> MQNNNEFKIGNRSVGYNHEPLIICEIGINHEGSLKTAFEMVDAAYNAGAEVVKHQTHIVEDEMSDEAKQVIPGNADVSIYEIMERCALNEEDEIKLKEYVESKGMIFISTPFSRAAALRLQRMDIPAYKIGSGECNNYPLIKLVASFGKPIILSTGMNSIESIKKSVEIIREAGVPYALLHCTNIYPTPYEDVRLGGMNDLSEAFPDAIIGLSDHTLDNYACLGAVALGGSILERHFTDRMDRPGPDIVCSMNPDTFKELKQGAHALKLARGGKKDTIIAGEKPTKDFAFASVVADKDIKKGELLSGDNLWVKRPGNGDFSVNEYETLFGKVAACNIRK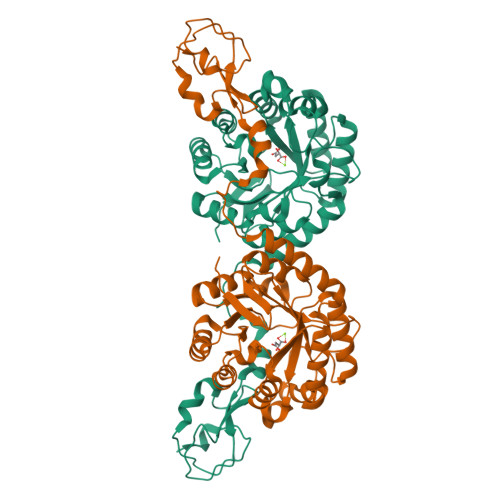GAQIKKTDIE N-BUTYL-N'-HYDROXYGUANIDINE 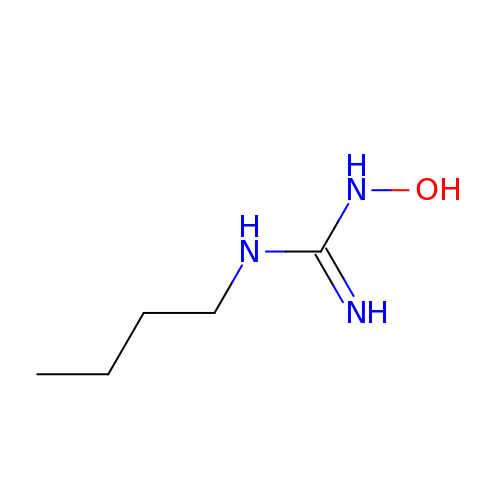| C5 H13 N3 O | ULDDTFAPYWLDGF-UHFFFAOYSA-N> MFIKPGRCPKPAVQEDFDAARYLGVW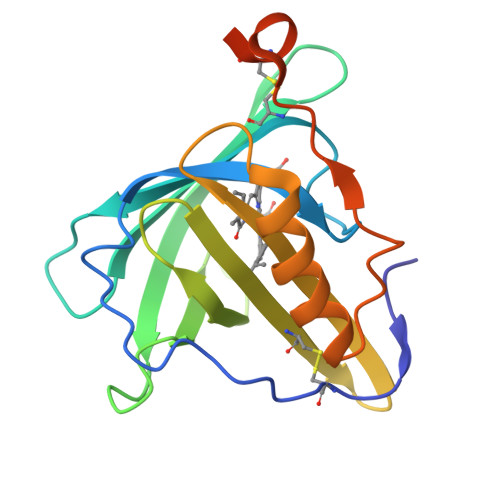YDIQRLPNKFQKGECATATYSLSPGEGFSVFNRERLANGTIKSVIGSAIAEDPCEPAKLQFFHENAAPVPYWVLSTDYDNYALVYSCINLGASHAAYASIVSRQPTLPEETIKKLQGTMSSFGVGVDTLLTTNQDAAYCSAMNQKLAAALEHHHHHH> AAQTNAPWGLARISSTSPGTSTYYYDESAGQGSCVYVIDTGIEASHPEFEGRAQMVKTYYYSSRDGNGHGTHCAGTVGSRTYGVAKKTQLFGVKVLDDNGSGQYSTIIAGMDFVASDKNNRNCPKGVVASLSLGGGYSSSVNSAAARLQSSGVMVAVAAGNNNADARNYSPASEP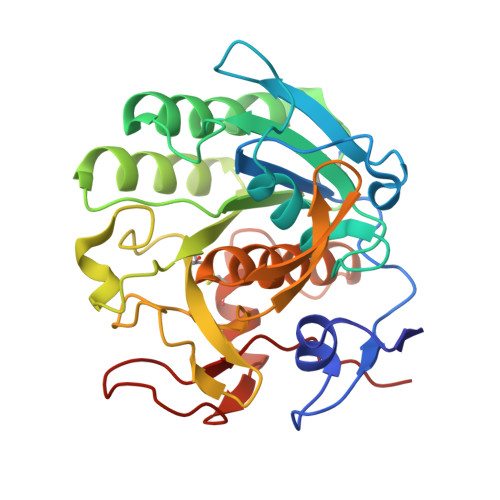SVCTVGASDRYDRRSSFSNYGSVLDIFGPGTSILSTWIGGSTRSISGTSMATPHVAGLAAYLMTLGKTTAASACRYIADTANKGDLSNIPFGTVNLLAYNNYQA>[2x]MRGSHHHHHHMQILLANPRGFCAGVDRAISIVENALAIYGAPIYVRHEVVHNRYVVDSLRERGAIFIEQISEVPDGAILIFSAHGVSQAVRNEAKSRD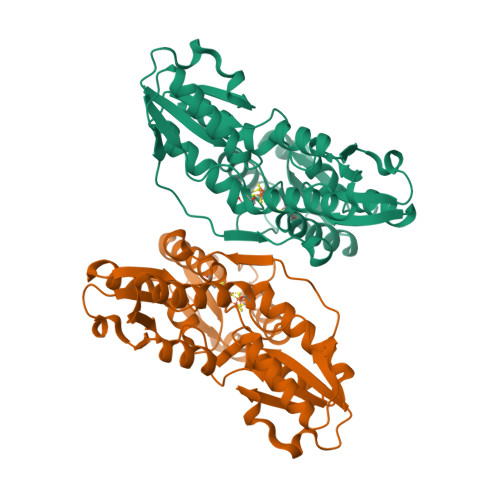LTVFDATCPLVTKVHMEVARASRRGEESILIGHAGHPEVEGTMGQYSNPEGGMYLVESPDDVWKLTVKNEEKLSFMTQTTLSVDDTSDVIDALRKRFPKIVGPRKDDICYATTNRQEAVRALAEQAEVVLVVGSKNSSNSNRLAELAQRMGKRAFLIDDAKDIQEEWVKEVKCVGVTAGASAPDILVQNVVARLQQLGGGEAIPLEGREENIVFEVPKELRVDIREVD>MKYNAPNTTPSSIGPQIRLDYYYKKALVDAAKEMYFGQLAEVTNMPKNMGKQIKLYHYVPLLDDRNVNDQGIDAAGATIANGNLYGSSKDIGTIPSKLPALTENGGRVNRVGFTRIQLIGSIKKFGFFYEWTQEAMDFDTDEELDSHLIQEAVKGANEITEDQLQIDLLNGAGVVRYPGAATSNADMTGEGTATVVTYEGLVKMGITLNDNLCPMQTKLIAGSLMTDTRTIQGARALYIGSELELQLRKMKDPFDNAAFIPVQQYADAGNLLKGEIGSIASFRVIVVPKMLKWAGAGATVTTNPGYYATSGKYDVFPMLCVGSGSFTTIGFQTDGKTVKFTTYTKKPGIETVSYADPYGEMGLTSIKWYYGSLILRPEWIALFKTVAAM[9x];>[9x]MAYSDVDAILADGKQAVAVKHGGGLVVVGELGAQVLAAKDVSELPDGVGGTAPGAATTTTAGVVKQSTTQAASVATDVAGVVTDLNALITKLKAAGIMA

We isolated and characterized two Shigella podophages that have notably different features when compared with classical podophages and instead are most closely related to phage N4. We describe the isolation and characterization of phages Moo19 and B2, including whole-genome sequencing and analysis, cryo–electron microscopy (cryo-EM) structure determination, mass spectrometry, host range studies, and enzymatic assays of the tail proteins. Our work shows that these phages have divergent decoration proteins and unique tail structures, and encode and package their own phage-dependent RNA polymerase, and the tails, which display esterase activity, are dependent on specific O-antigen modifications of lipopolysaccharide (LPS) for entry. Moo19 and B2 are similar to bacteriophage N4—these are all T = 9 podophages, which encapsidate their own polymerases—a hallmark of this phage family.

We also analyzed the data by imposing icosahedral symmetry to visualize the capsids at high resolution (3.6 and 3.4 Å for Moo19 and B2, respectively). Both capsids have a T = 9 geometry (see Fig. 2B for a depiction of the capsid proteins that comprise the asymmetric unit). The major capsid protein of each has the HK97-like fold that is present in most, if not all, dsDNA tailed phages. Using DALI, both the major capsid proteins of Moo19 and B2 are most similar to Ralstonia phage GP4 (37), another T = 9 podophage with an RMSD (root mean square deviation) of 3.0 and 3.2 Å, respectively. The decoration proteins of both Moo19 and B2 bind the capsid proteins at the same quasi-sixfold symmetry axes in both phages but have notably different folds. By contrast, B2’s decoration protein (gp45) is only 99 amino acids. It also forms a homotrimer but is quite unlike Hoc or gp28. To our knowledge, there are no reported phage structures that have structural homology to B2’s gp45. However, B2’s gp45 had poor alignment with these helical decoration proteins and did not share a recognizable topology.> MASGWSDFRADPVIVNQDVVVFGNVFVDYLIGNASEMTGAADFVPGNVVNVNIIGNTVSTFVKSDVLMGDTITIDGNITATRLYGDASNMSGLPTLPPNANIDMVGNIVANTNTNKFVSVDTFTGDVTTNVATISNANVGTVTTNTTFFGNVITNVFNIGNLILTSSNVDTLNVTSLVASNVVSSQVDVQATIANSDLNVTRFDATSISAEIFVSSETLAVSNITNLIANIANIQGTTTVTGNLVGNIANVNTLTGNVTGNLFFTNLIIGNITANIFNTTTANVSNLITSNVSASNVSASNVTSTLFTIGNLNTNVATISNLFVTGTTIAGNTTFSSFSVSSLVANISGNNASIPTFTPNVLSTSNITIDGNAVVTGNAGFRTLNVTSLTANVLTTRGDVSNLYTDVINVNTNVFISSANILANNVITVQMNNISNVNITGNAEAFDVSANSVLMSTLSVGGILSLGNVNTNDISFGNIVTGNFFANFANVGNVQ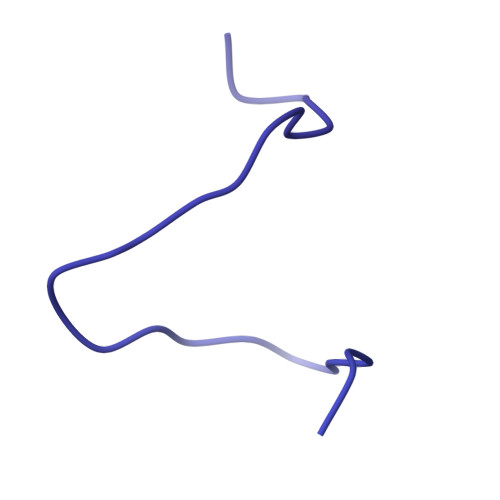GNANVITMYSTTLTSNSAQIGNISGFSIVSNLGNAVSMFVGNLNTGTLVANNSTVGNITYISGNIGNANAQTVRVSGLLSASGVALTFNSITSNVAGNSLTVHGNLRTNSVTTEILTGNVGNLSILNTGNLFANSISVGQSFVISNFANAFIISSQTTNASVITANISGNIRVTNTLEANVVNSDSANIIIKNVSTSGNVSNTFTTGNLTVTNAVFRSGITGNNIEVVGNVNCDGNTTVTTLSYGNLITSVYNTRNIFGNITANTVNITNSNIGNVVTSNINANSLIITNLIPTVDITANVLRASQVNTGWFYGNATCNVLSMSNSVSINTLLSAEVFTSETINANANVSVATINSLGNTVAISRPSFLGNANIRLVISNVITIGNLTANTLVGDSFTATGIVNAINSNSQSDSIATNVTGNIIIRGNLILASSASAQSNASVFNPTNLISLNANSLSSLTATNVSANNVVISNTWQVSNLIVSNISAPNVTANSFQAISMTGRYYRPGISIERAGNLIVSNSLTSTANILQVLTSNTGQVNITNTMFGNISMSNIIVTGVVVTGNLTMGNVIANAVTTSVSTITGNATFGNLTVTDAVIIRGNITANNISTGSYIYGNGAFITGNLTSSGNANISIATRMFGTNSAINVAGTFTGVGNTNTTNATIANLTTNTLLSIGNLSTTGNFTVNSLSVGNLFANGSTIQLSNLANIQVSNLIYSGNVVVSNLSANTLSYVQNIGTSTQLQSGTMNVNNILSAGRFRLSISSTAPVFAGWTMGRVSLSGQSLRTNSGNPRTITFTTPLPAGYSYGIQLSVYSTVFGQTMALFNITVVSLTNTSVQFYIWNNPGGSGDSNTYIGYFAYAY>[8x]SNAPVNQVQSSVSWPQNGSLNSVSAPLMSYTPISFDAKIPVASVDKLRKDQDLILGTLPANSEDAGARGLFVRANDDGLQITSHGELVLDLSKRELAQLPA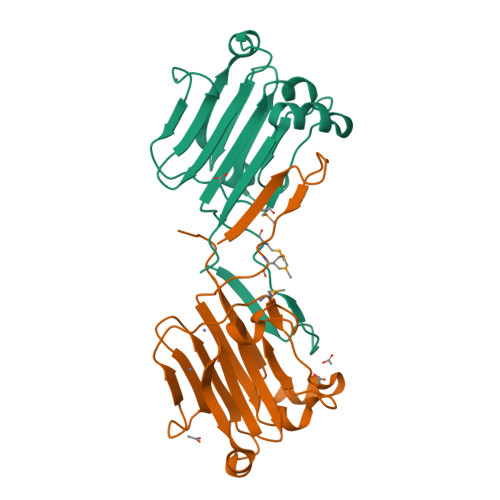DATIAISATEDETTAGIEGDDSTTETVERDVRPIIMGIYTELESNAAADLLNAGLNAHVEINSRFTSSPTLAKYAS>[2x]GSHMHESKEWYHASLTRAQAEHMLMRVPRDGAFLVRKRNEPNSYAISFRAEG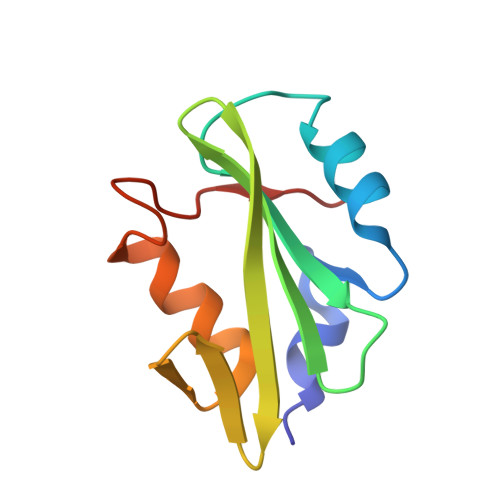KIKHCRVQQEGQTVMLGNSEFDSLVDLISYYEKHPLYRKMKLRYPINEE>TTGHSYEKYNNWETIEAWTKQVTSENPDLISRTAIGTTFLGNNIYLLKVGKPGPNKPAIFMDCGFHAREWISHAFCQWFVREAVLTYGYESHMTEFLNKLDFYVLPVLNIDGYIYTWTKNRMWRKTRSTNAGTTCIGTDPNRNFDAGWCTTGASTDPCDETYCGSAAESEKETKALADFIRNNLSSIKAYLTIHSYSQMILYPYSYDYKLPENNAELNNLAKAAVKELATLYGTKYTYGPGATTIYPAAGGSDDWAYDQGIKYSFTFELRDKGRYGFILPESQIQATCEETMLAIKYVTNYVLGHL[3x];>[3x]KKVYAF

The carboxypeptidase TAFIa (activated thrombin activatable fibrinolysis inhibitor) is a central player in fibrinolysis. TAFIa removes carboxy-terminal lysines and arginines from partially degraded fibrin. Carboxypeptidase B (CPB) was used instead of TAFIa for practical reasons, since TAFIa was found to be highly unstable with a half-life of approximately 2h at 22 °C30. CPB, on the other hand, is stable and highly homologous to TAFIa with 48% sequence identity.

In addition, we obtained crystal structures of the complexes of anabaenopeptin B (1), anabaenopeptin C (2) and anabaenopeptin F (3) with the surrogate protease carboxypeptidase B (CPB). The general binding modes of 1–3 were found to be very similar and in the following discussion the complex with 2 is used as an example. The linear part of the anabaenopeptins, which mimics the carboxy-terminus of the TAFIa substrate fibrin, deeply penetrated the active site channel and bound in the carboxylate- and specificity-pockets, while the circular parts of the anabaenopeptins were positioned in the entrance of the channel and completely blocked the channel like a plug, thereby preventing other molecules from entering it. Calculations with PISA33 revealed that the total surface area of 2 was 1036 Å3, while the area of the 2–CBP interface was 519 Å3. Thus, about 50% of the surface of 2 got buried upon binding, contributing to the high affinity. In line with the very high binding affinity of 2, there were no unsatisfied buried hydrogen bonds. All hydrogen bond donor and acceptor atoms of 2 interacted either with hydrogen bond donor/acceptors from the protein, or with bound water molecules. Within the cyclic core of 2, the side chain of the D-lysine residue (R2) had van der Waals interactions with the side chains of Tyr198 and Phe279. The amide moiety bridging R2-D-lysine and R3-valine interacted with the side chains of Arg71, Arg127 and Tyr248. Finally, a van der Waals contact was present between the R4-homotyrosine side chain of the anabaenopeptin and the side chain of Met125.>MASEVVSFSFTKFNPNPKDIILQGDALVTSKGKLQLTKVKDGKPVDHSLGRALYAAPIHIWDDSTDRVASFATSFSFVVEAPDESKTADGIAFFLAPPDTQPQKDGGFLGLFNDSNKSIQTVAVEFDTFSNTWDPSARHIGINVNSIESMKYVKWGWENGKVANVYISYEASTKTLTASLTYPSNATSYIVSANV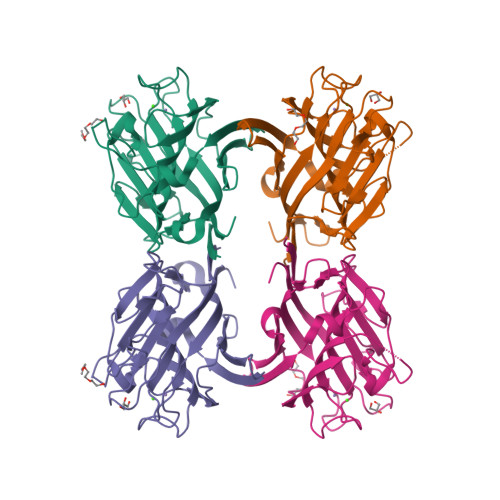DLKSALPEWVRVGFSATSGLSRDHVETHDVLDWSFTSTLQAPSDDSNLEHHHHHH[2x]> RSMEEETHTDAKIRAENGTGSSPRGPGCSLRHFACEQNLLSRPDGSASFLQG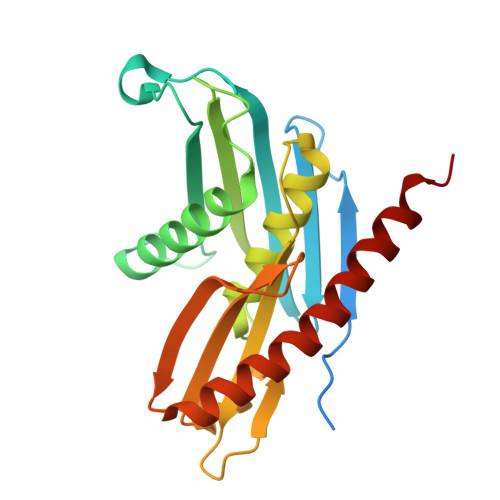DTSVLAGVYGPAEVKVSKEIFNKATLEVILRPKIGLPGVAEKSRERLIRNTCEAVVLGTLHPRTSITVVLQVVSDAGSLLACCLNAACMALVDAGVPMRALFCGVACALDSDGTLVLDPTSKQEKEARAVLTFALDSVERKLLMSSTKGLYSDTELQQCLAAAQAASQHVFRFYRESLQRRYSKS> VDEQPLENYLDMEYFGTIGIGTPAQDFTVVFDTGSSNLWVPSVYCSSLACTNHNRFNPEDSSTYQSTSETVSITYGTGSMTGILGYDTVQVGGISDTNQIFGLSETEPGSFLYYAPF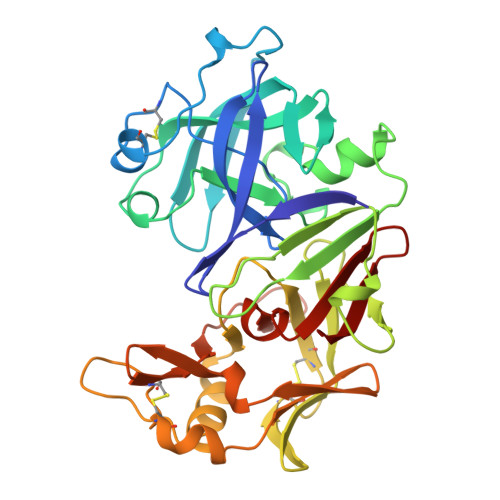DGILGLAYPSISSSGATPVFDNIWNQGLVSQDLFSVYLSADDQSGSVVIFGGIDSSYYTGSLNWVPVTVEGYWQITVDSITMNGEAIACAEGCQAIVDTGTSLLTGPTSPIANIQSDIGASENSDGDMVVSCSAISSLPDIVFTINGVQYPVPPSAYILQSEGSCISGFQGMNVPTESGELWILGDVFIRQYFTVFDRANNQVGLAPVA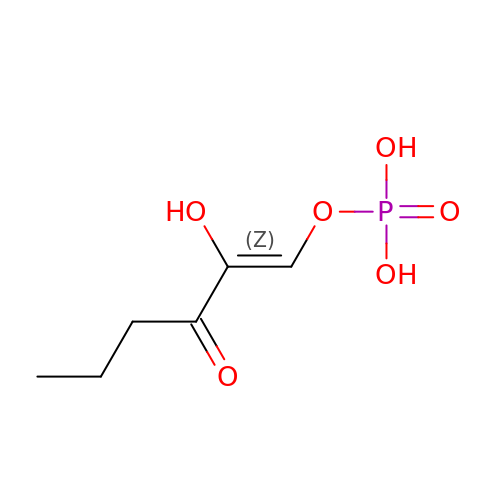(1Z)-2-HYDROXY-3-OXOHEX-1-EN-1-YL DIHYDROGEN PHOSPHATE | C6 H11 O6 P | HEBDCWKDNSCZMW-XQRVVYSFSA-N4-(5-{[(2-chloropyridin-4-yl)methyl]carbamoyl}thiophen-2-yl)-1-benzothiophene-2-carboxamide | C20 H14 Cl N3 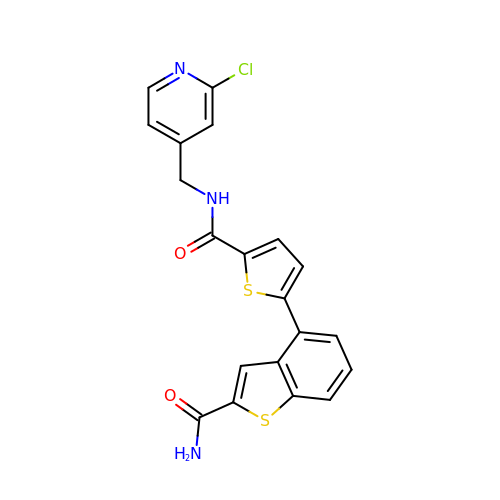O2 S2 | SKAFXNGFXPGQIG-UHFFFAOYSA-N6-{[(1S)-1-(4-chlorophenyl)ethyl]amino}-1-cyclopentyl-1,5-dihydro-4H-pyrazolo[3,4-d]pyrimidin-4-one 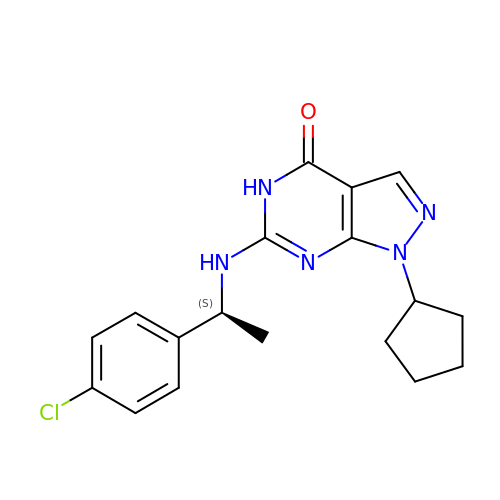| C18 H20 Cl N5 O | FIUCLBJMUGCQTF-NSHDSACASA-N>MSPILGFWKIKGLVQPTRLLLEYLEEKYEEHLYERDEGDKWRNKKFELGLEFPNLPYYIDGDVKLTQSMAIIRYIADKHNMLGGCPKERAEISMLEGAVLDIRYGVSRIAYSKDFETLKVDFLSKLPEMLKMFEDRLCHKTYLNGDHVTHPDFMLYDALDVVLYMDPMCLDAFPKLVCFKKRIEAIPQ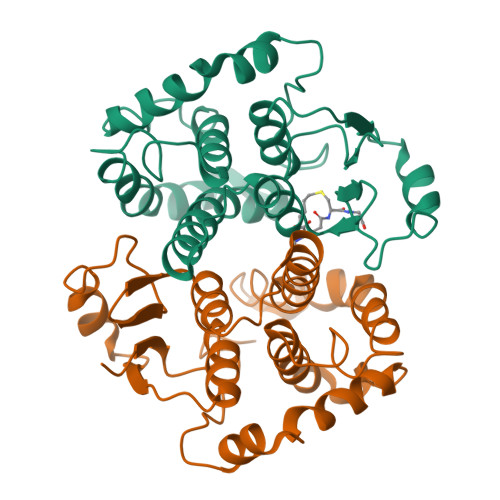IDKYLKSSKYIAWPLQGWQATFGGGDHPPK[2x]> VNKERTFLAVKPDGVARGLVGEIIARYEKKGFVLVGLKQLVPTKDLAESHYAEHKERPFFGGLVSF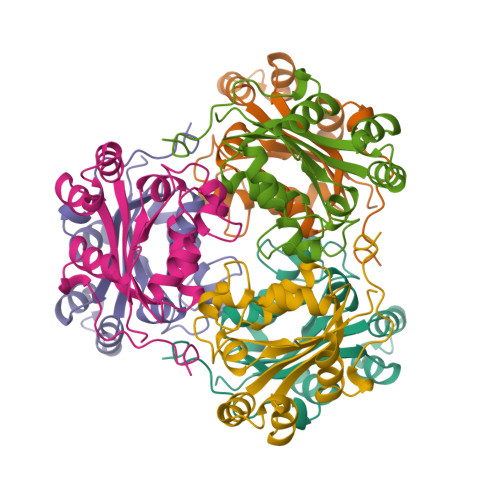ITSGPVVAMVFEGKGVVASARLMIGVTNSLASAPGSIRGDFGVDVGRNIIHGSDSVESANREIALWFKPEELLTEVKPNPNLYE> AHHHHHHGSNPFHDLEPGPDVPEVVYAIIEIPKGSRNKYEL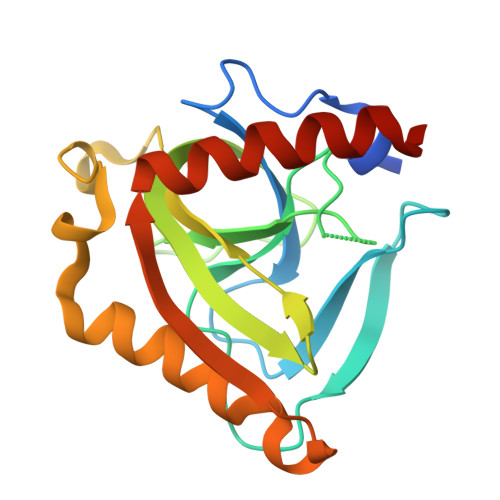DKKTGLLKLDRVLYSPFFYPVDYGIIPRTWYEDDDPFDIMVIMREPVYPLTIIEARPIGLFKMIDSGDKDYKVLAVPVEDPYFKDWKDIDDVPKAFLDEIAHFFKRYKELQGKEIIVEGWEGAEAAKREILRAIEMYKEKFGKKE>MEIARTNKNSVVKYVPAAVGAAYQMGKSIVPYAPTIVDALGNVVSRATGRKKKSKGKEVQNQIVGGIGAIAAPVSITKRVRGMRPSFRQTKGKVHIVHRELVTSVINLVGNFRVNNNVSAQIGQFRINPSNSSLFTWLPTIASNFDSYRFTSIRFVYVPLCATTETGRVSLFWDKDSQDPLPVDRAALSSYGHSNEGPPWAETTLNVPTDGKQRFVTDSNTTDRKLVDLGQFAFATYAGGSNNQIGDIYVEYGVEFSEAQPAGGLTQYITKSVGATASTTGPSYVVDANIN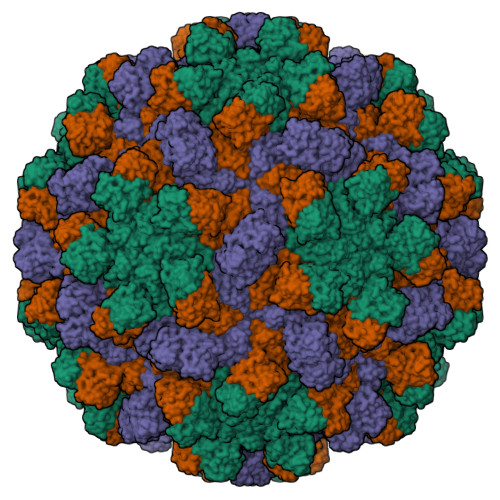VNATTANVEFFSPGTFLITAVVYGSTIASPSMAGGNGTLIGDLPVVGGSNASIWTCVFSTTGVSTSVPTFTQAGTGLTRVQYTITRVNSQTAYQV[3x]> MPSDILVVAALGRPFTLGMLYDARNDKLIPGFTLWEDEVIEESTLESSQPSSAFEIIASDSTDDKSSLMDIEASLKASFLGGLVEVGGSAKYLNNQKKFKNQSRVTLQYKATTSFKQLMTNLGTKHVEYSELFENIQATHVVIGILYGANAFFVFDSNKVDSTNVQEIQGQMEAVIKKIPSVEISGKASVQLTGEETDITNSFSCEFHGDFFLTTNPTTFEDAVKTYQQLPQMMGKDNAVPMTVWLVPMVNFYSEAPQLMADSSTPILRKVRNTLEAIVQVQMRCNDALDDPTVNLFTEVQKKLSDFQKICDDHMSKLQATIAKKLFAIRSGDEDESALLNLFEENLQSPFNIESLNMWMEFEEREINVLRSCMDILTKAKPKVIFNQGVLFKGLYDSKVKHALCYVFTNVTKNDVFLNVLNEFLDSPQSRPKKLRPSPKDYWYSYDDIPETMREKAYLFRNLAKEMNNRCVHFFVTAIHNPKQEGAGIHYYRESIQIIDEFTKPYMPGVESIKDRRELQWYDCELTLDPETAHQVLTLSEGNKKAVSGNTKSPTDHLEKFSHFQQVMCTKGLSGRHYWELEWSGYVGAGVTYKGIGRKTSTSDSSLGKNEKSWLFEYS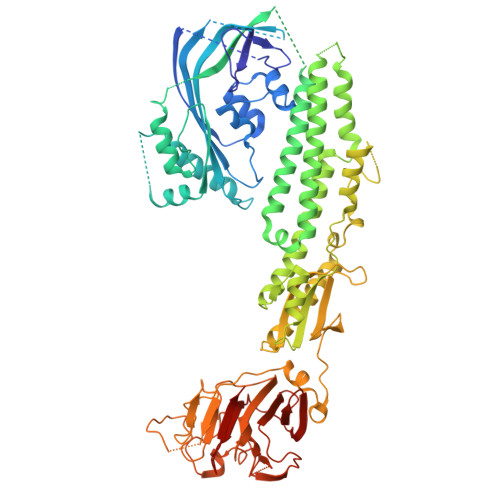TKSGYQQIHNSKKTRVTVSSTGFKLLGVYLDWPAGTLSFYMVNKAWVTHLHTFHTKFNEAVYPAFLIGDAQQKVNGQIKLL>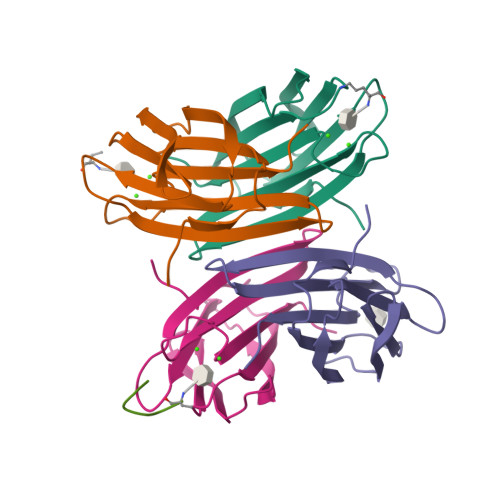[4x]MATQGVFTLPANTRFGVTAFANSSGTQTVNVLVNNETAATFSGQSTNNAVIGTQVLNSGSSGKVQVQVSVNGRPSDLVSAQVILTNELNFALVGSEDGTDNDYNDAVVVINWPLG;>KAAKACX[3x]>GSMNVILSIDQSTQSTKVFFYDEELNIVHSNNLNHEQKCLKPGWYEHDPIEIMTNLYNLMNEGIKVLKDKYTSVIIKCIGITNQRETVIIWDRITGKPLYNAIVWLDTRVEELVTEFSAKYNNNDIQKKTGTYFNTYFSAFKILWLIQNNPEIKQKIDDGTAVIGNINTWLIFNLTKGNCYTDVTNASRTLLMDINTLQWDEKMCKIFNITNMSVLPEIKSNCSNFGLVKSEHVPDYLNIPITGCIGDQQSACIGQAIFDEGEAKCTYGTGVFLLINTGEKVVYSTCGLITTICYKFNDNDKPKYALEGSIGTAGSGVSWLLKNKLIDDPSEASDIMEKCENTTGVIFVPAFSGLYAPRWRSDARASIYGMTFNTERSHIVRALLEGIAFQLNEIVDSLTSDMGIEMLHVLRCDGGMTKNKPFMQFNSDIINTKIEVSKYKEVTSLGAAVLAGLEVKIWDSLDSVKSLLRRSDAVFHSKMDDKKRKKKTSEWNKAVERTLIQL[4x]

GK catalyses the rate-limiting step of glycerol utilization, with phosphorylation serving to sequester the sugar in the cell. The 501-residue GK polypeptide is arranged as two domains separated by a deep cleft. Each domain is constructed around a βββαβαβα core that is characteristic of the sugar kinase/Hsp70/actin superfamily of proteins. In agreement with gel filtration experiments (data not shown), PfGK is a dimer in the crystal.

The crystal structure of PfGK in complex with glycerol was solved by molecular replacement using EcGK as a search model. The structure was refined against data extending to 1.5 Å spacing to give a final model that agrees well with the X-ray terms. Glycerol is defined by electron density deep in the cavity between the domains. Its hydroxyl groups fulfil their hydrogen bonding potential through charge–dipole interactions with Glu84, Arg83 and Asp246 and dipole–dipole interactions with Arg83, Tyr135 and Gln247. The C3-OH of the glycerol forms hydrogen bonds to two water molecules that occupy a narrow channel to the protein surface. The apolar face of the glycerol moiety packs against the side-chains of Trp103 and Phe271, the latter representing the only glycerol-binding residue contributed by domain II. The pattern of interactions is similar to that in glycerol complexes of bacterial GKs. Residue Tyr354, whose hydrophobic nature is conserved among eukaryotic GK sequences, occludes the alternate conformer of Tyr135 in the closed form of the enzyme. In PfGK, the β11-β12 loop (residues 227–238) corresponding to the glycine-rich loop in EcGK is well defined in the electron density maps. In contrast to the exposure of these loops in EcGK, in PfGK this loop is oriented towards the core of the dimer, an orientation that would sterically hinder tetramer formation.As members of the Caliciviridae family, norovirus virions consist of an approximately 7.5-kb positive-sense single-stranded RNA genome linked at its 5′ end to a viral protein (VPg). This genomic RNA is enclosed within a nonenveloped, T = 3 capsid approximately 40 nm in diameter. The capsid is formed from 90 dimers of the major structural protein, VP1, in one of three quasiequivalent conformational states: A-type VP1 proteins make up the icosahedral 5-fold axes and form AB dimers with B-type VP1 proteins, whereas C-type VP1 proteins form CC dimers at 2-fold axes. Each VP1 monomer comprises an N-terminal region, a shell (S) domain, and a protruding (P) domain (subdivided into proximal [P1] and distal [P2] subdomains). P domains extend outward from this shell and mediate interactions with receptor molecules and cofactors such as bile salts.

We used cryo-electron microscopy (cryo-EM) to determine the structure of wtMNV at 3.1-Å resolution. wtMNV was cultivated in RAW264.7 cells, then purified by ultracentrifugation through a sucrose cushion and 2 sucrose gradients before being applied to lacey carbon grids and vitrified. The P domains from AB-type dimers (surrounding the icosahedral 5-fold axes) are rotated approximately 100° clockwise relative to their position in the published structure, whilst the P domains from CC-type dimers (at icosahedral 2-fold axes) are rotated approximately 75° anticlockwise. The P domains are also located much closer to the shell of S domains (separated by approximately 6 Å rather than approximately 16 Å). Interestingly, the positioning and orientation of the P domains in our map of apo MNV are closer (although not identical) to recent structures of bile-complexed MNV, despite the lack of bile salts. The quality of the data allowed us to build a hybrid atomic model for VP1. The resolution in the S domain was sufficient to allow confident building of most residues up to the flexible linker region. As expected, the flexible linker connecting the S and P domains was not resolved for A- or B-type VP1. However, the flexible linker for C-type VP1 was resolved, suggesting it is less mobile than the A- or B-type conformer, which correlates with the improved resolution of C-type P domains. Most of the C-type VP1 N-terminal region is disordered (residues 1–29), whereas A- and B-type VP1 N-terminal regions are better resolved (missing residues 1–19 and 1–16, respectively) and have distinct conformations. Using focussed 3D classification, we identified a remarkable diversity in P domain dimer positioning that was not coordinated over the capsid surface and was not equal between different quasiconformers, with CC-type dimers being less mobile than AB-type dimers.

>[3x]MRMSDGAAPKANGSEASGQDLVPAAVEQAVPIQPVAGAALAAPAAGQINQIDPWIFQNFVQCPLGEFSISPRNTPGEILFDLALGPGLNPYLAHLSAMYTGWVGNMEVQLVLAGNAFTAGKVVVALVPPYFPKGSLTTAQITCFPHVMCDVRTLEPIQLPLLDVRRVLWHATQDQEESMRLVCMLYTPLRTNSPGDESFVVSGRLLSKPAADFNFVYLTPPIERTIYRMVDLPVIQPRLCTHARWPAPVYGLLVDPSLPSNPQWQNGRVHVDGTLLGTTPISGSWVSCFAAEAAYEFQSGTGEVATFTLIEQDGSAYVPGDRAAPLGYPDFSGQLEIEVQTETTKTGDKLKVTTFEMILGPTTNADQAPYQGRVFASVTAAASLDLVDGRVRAVPRSIYGFQDTIPEYNDGLLVPLAPPIGPFLPGEVLLRFRTYMRQIDTADAAAEAIDCALPQEFVSWFASNAFTVQSEALLLRYRNTLTGQLLFECKLYNEGYIALSYSGSGPLTFPTDGIFEVVSWVPRLYQLASVGSLATGRMLKQ>[4x]GSSGAFEDRDPTQFEERHLKFLQQLGKGNFGSVEMCRYDPLQDNTGEVVAVKKLQHSTEEHLRDFEREIEILKSLQHDNIVKYKGVCYSAGRRNLKLIMEYLPYGSLRDYLQK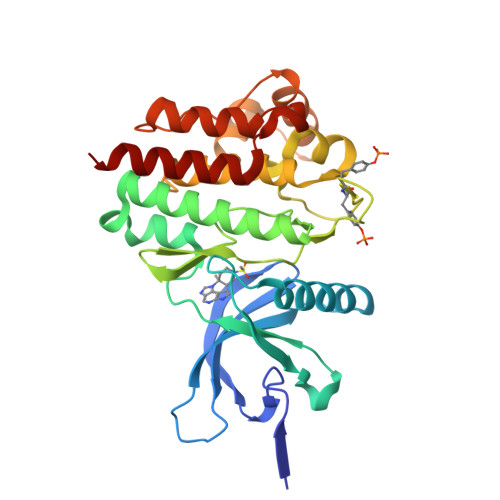HKERIDHIKLLQYTSQICKGMEYLGTKRYIHRDLATRNILVENENRVKIGDFGLTKVLPQDKEYYKVKEPGESPIFWYAPESLTESKFSVASDVWSFGVVLYELFTYIEKSKSPPAEFMRMIGNDKQGQMIVFHLIELLKNNGRLPRPDGCPDEIYMIMTECWNNNVNQRPSFRDLALRVDQIRDNMAG> GAMGSMSRIDSDLQKALKKACSVEETAPKRKHVRACIVYTWDHQSSKAVFTTLKTLPLANDEVQLFKMLIVLHKIIQEGHPSALAEAIRDRDWIRSLGRVHSGGSSYSKLIREYVRYLVLKLDFHAHHRGFNNGTFEYEEYVSLVSVSDPDEGYETILDLMSLQDSLDEFSQIIFASIQSERRNTECKISALIPLIAESYGIYKFITSMLRAMHRQLNDAEGD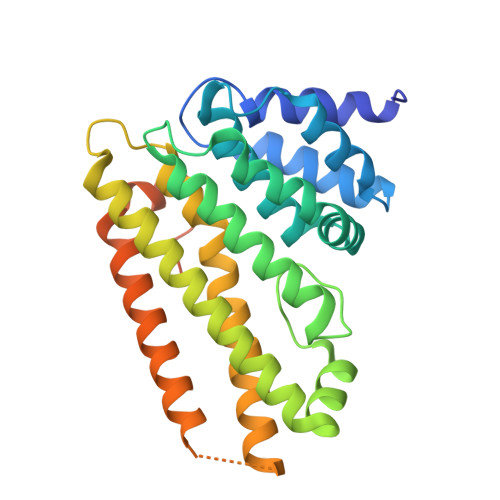AALQPLKERYELQHARLFEFYADCSSVKYLTTLVTIPKLPVDAPDVFLINDVDESKEIKFKKREPSVT(5aS,12aS,13aS)-9-bromo-12,12-dimethyl-2,3,11,12,12a,13-hexahydro-1H,5H,6H-5a,13a-(epiminomethano)indolizino[7,6-b]carbazol-14-one | C21 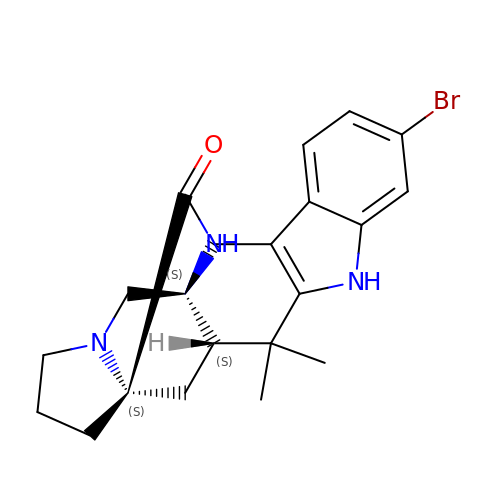H24 Br N3 O | LMABZAWQQDGLLN-DQLDELGASA-N> MASMTGGQQMGRDEAGITGTWYNQLGSTFIVTAGADGALTGTYESAVGNAESRYVLTGRYDSAPATDGSGTALGWTVAWKNNYRNAHSATTWSGQYVGGAQARINTQWLLTE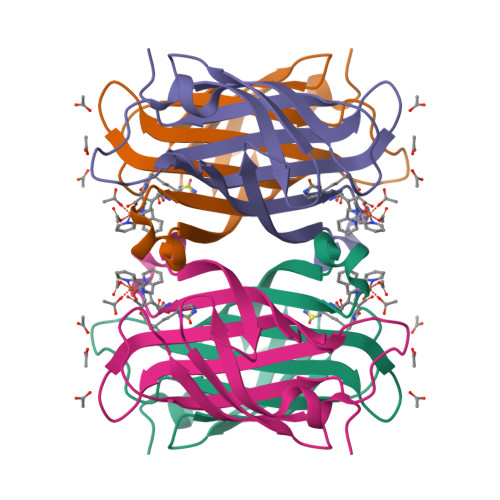GTTEANAWASTLVGHDTFTKVKPSAASIDAAKKAGVNNGNPLDAVQQ>MITKSNEFWTPKRLLETDDRIFLVVGGRGVGKTFNVTGEALDDLFFNNVSMVYLRRLGVEIDELEKNNFITEEMLRVYFGNRFSDFNADESKQIMRFSIDGAIHEIKAIRNKIFFDDRCIVYFIALSRAGHVKSNNYPDVKYLVFDEVIIDRSIMPNARYIRNEFTVLLNLIETIKRKREDFYLFMLSNVGENFNPIFAGLGYYLTHEDIKKGFVKREDYCVQFVENKQEELNMTDPFVRLGAKNRDFSNSKTNAFENIRTPYFKHYGKKPKLLVKYDRQYLGIAERKIPSGLEYYYQVYKTLDGLENITVFNNNFDTLMEDEVFLEETQLKKKFKTYFELFQQNMVYHESPETFLEWSKFVYALKLEHHHHHH[5x]

We present the first atomic-resolution crystal structure of a multimeric ring form of a viral dsDNA packaging motor, the ATPase of the asccφ28 phage, and characterize its atomic-level dynamics via long timescale molecular dynamics simulations. In contrast, a close homolog of the φ29 ATPase from the related bacteriophage asccφ28 (gp11) has been shown to form highly soluble functional rings; extensive analytical ultracentrifugation and small-angle X-ray scattering experiments show that the ATPase forms pentameric rings in solution. Individual subunits within the ring are organized into two globular domains connected by a linker domain, each of which is nearly identical to the corresponding domains of the φ29 gp16. Like φ29 gp16, the N-terminal domain adopts the canonical ASCE ATPase fold, while the C-terminal domain is a ‘vestigial nuclease domain’.

Two crystal forms of gp11 were obtained: (i) tetragonal crystals belonging to space group P43212 and (ii) trigonal crystals belonging to space group P3221. While the three structures described here were determined in the absence of nucleotide, the active sites of ASCE ATPases are well characterized and can be accurately identified. Two distinct conformations of the Walker A motif are apparent in our crystal structures. One conformation binds either a SO42− or PO43− ion in the canonical β-phosphate position. The ion forms hydrogen bonds with the backbone of the Walker A motif in lieu of a β-phosphate, typically provided by ATP or ADP, which explains why the Walker A backbone adopts a conformation similar to a typical nucleotide-bound ATPase configuration. However, because the structure was solved in absence of nucleotide or nucleotide analog, it lacks any interactions mediated by the α- and γ-phosphates, ribose sugar, or adenosine base. Thus, this structure likely represents a conformation with mixed characteristics from both the apo and nucleotide-bound configurations. However, the crystal structure of asccφ28 gp11 ring reported here shows no such helicity in the N- or C-terminal domains. We suspect that we do not observe helicity in the crystal structures due to lack of substrate DNA imparting helicity.Ankyrins are a family of scaffold proteins which play essential roles in connecting numerous ion channels, cell adhesion molecules, and receptors to the spectrin-based cytoskeleton beneath membranes and thereby provide mechanical support for plasma membranes and control the activities of excitable tissues including neurons and muscles. There are three members in the human ankyrin family: ankyrin-R/B/G (AnkR/B/G) encoded by ANK1/2/3, respectively. They all consist of a highly similar N-terminal membrane binding domain composed of 24 ankyrin (ANK) repeats, a spectrin-binding domain comprised of two ZU5 domains, and a UPA domain followed by a death domain (DD) and a variable C-terminal regulatory domain. The wide-ranging physiological functions of ankyrins are the result of ankyrin's remarkable capacity for binding to and anchoring numerous membrane targets, via their N-terminal 24 ANK repeats, to specific membrane micro-domains in coordination with spectrin-based cytoskeletal structures. The 24 ANK repeats of ankyrins form a superhelical solenoid with an extremely conserved elongated inner groove, which contains multiple quasi-independent target binding sites.

Using isothermal titration calorimetry (ITC)-based quantitative binding assays, we identified a 48-residue auto-inhibitory segment (residues 1577–1624, referred to as ‘AS’) as the complete ANK repeat-binding region. After extensive trials of screening and optimization, we succeeded in obtaining good-diffraction crystals of AnkR_AS fused at its C-terminus with the AnkB_repeats and solved the structure of the fusion protein at 3.5 Å resolution. The residues connecting AS and ANK repeats (10 residues in total, ‘GSLVPRGSGS’) are flexible, indicating that the fusion of the two chains together does not introduce obvious conformational restraints to the complex. The 24 ANK repeats form a left-handed helical solenoid with each repeat rotating anti-clockwise by ∼16°. The inner αA helices and the finger loops of the 24 repeats line together to form an elongated concave inner groove, and the αB helices of the repeats form the solvent-exposed convex outer surface. The ANK repeats superhelix has outer and inner diameters of approximately 60 Å and 45 Å, respectively, and a total height of ∼150 Å. In the complex, AS adopts a highly extended structure binding to part of the inner groove formed by the N-terminal 14 ANK repeats (R1–14) with its chain orientation anti-parallel to that of ANK repeats. A 10-residue segment of AS (residues 1592–1601) forms an α helix when bound to ANK repeats. The binding of AS to ANK repeats can be divided somewhat arbitrarily into three sites (sites 1, 2, and 3) formed by the repeats 2–6, 7–10, and 11–14, respectively. The interactions in site 2 are mediated both by hydrophobic and hydrogen bonding interactions, while interactions in site 3 are mainly hydrophobic.

> GPGSEFCADQYWNEVAVIDAIPLAATEHDTMLEMSDMQVWSAGLTPSLVTAEDSGSLVPRGSGSKSDSNASFLRAARAGNLDKVVEYLKGGIDINTCNQNGLNALHLAAKEGHVGLVQELLGRGSSVDSATKKGNTALHIASLAGQAEVVKVLVKEGANINAQSQNGFTPLYMAAQENHIDVVKYLLENGANQSTATEDGFTPLAVALQQGHNQAVAILLENDTKGKVRLPALHIAARKDDTKSAALLLQNDHNADVQSKMMVNRTTESGFTPLHIAAHYGNVNVATLLLNRGAAVDFTARNGITPLHVASKRGNTNMVKLLLDRGGQIDAKTRDGLTPLHCAARSGHDQVVELLLERGAPLLARTKNGLSPLHMAAQGDHVECVKHLLQHKAPVDDVTLDYLTALHVAAHCGHYRVTKLLLDKRANPNARALNGFTPLHIACKKNRIKVMELLVKYGASIQAITESGLTPIHVAAFMGHLNIVLLLLQNGASPDVTNIRGETALHMAARAGQVEVVRCLLRNGALVDARAREEQTPLHIASRLGKTEIVQLLLQHMAHPDAATTNGYTPLHISAREGQVDVASVLLEAGAAHSLATKKGFTPLHVAAKYGSLDVAKLLLQRRAAADSAGKNGLTPLHVAAHYDNQKVALLLLEKGASPHATAKNGYTPLHIAAKKNQMQIASTLLNYGAETNIVTKQGVTPLHLASQEGHTDMVTLLLDKGANIHMSTKSGLTSLHLAAQEDKVNVADILTKHGADQDAHTKLGYTPLIVACHYGNVKMVNFLLKQGANVNAKTKNGYTPLHQAAQQGHTHIINVLLQHGAKPNATTANGNTALAIAKRLGYISVVDTLKVVTEEVTTTTTTITEKHKLNVPETMTEVLDVSDEEGDDTMTGDGGEYLRPEDLKELGDD> GMDFLTSTLLSGILYDGFKNGVAITTGFLKEK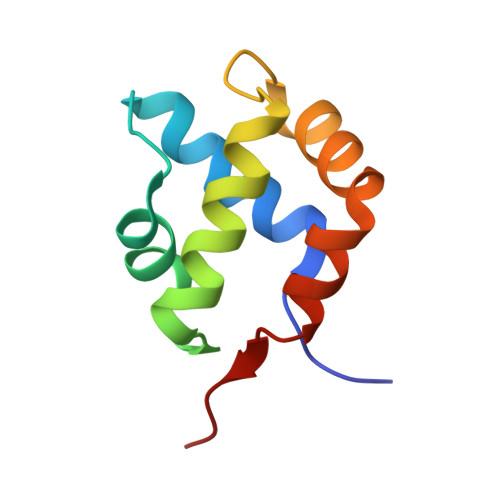LHGWIVDDTLLETLAYKVNTLELKDYGEHVIERKLNESSEIQQILKLIQPEQN> MQRSTRIVMAPFKSVLRRHKHHPEGLPLYNDMSKQWLCREGERWWLLDARGEQLPRVAAVAAQYITGQHRPDFTPGMITGDHVVIVNIKDVVMVGDQWIRVPITWQTAYPGGKYRIRLTDMYERDPCMLMWWFLKDEVNRHFVRKLKTRIAPLEKAWLYEDSIHPHADKNPRPLCWTDPEVKGWKYRDPQFIRRWKPNEF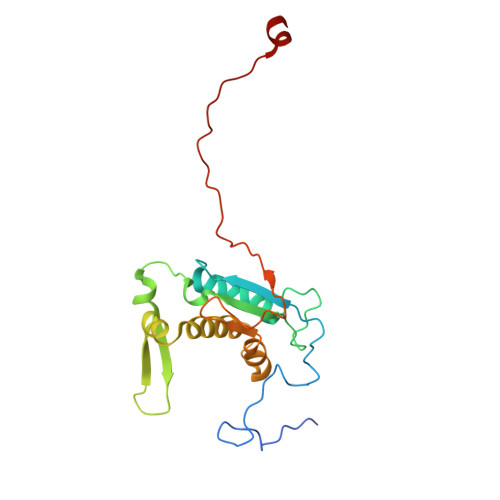MH>NQGVTRQRQQTKVFKLVSTYDKVAVKNAIRAAYRQVFERDLEPYIINSEFTALESKLSNNEINVKEFIEGLGTSELYMKEFYAPYPNTKVIEMGTKHFLGRAPLNQKEIQQYNQILASQGLKAFIGAMVNGMEYLQTFGEDTV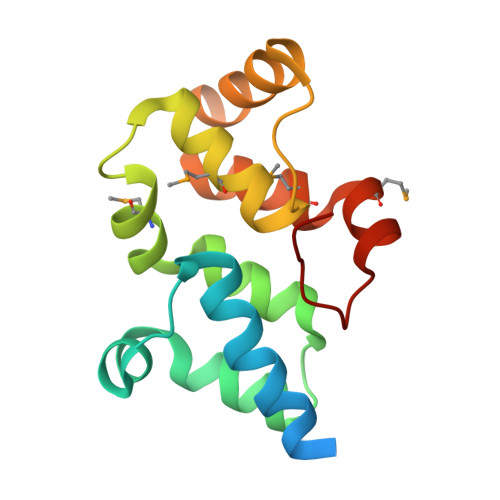PYRRF[2x]>MGSVLSTDSGKSAPASATARALERRRDPELPVTSFDCAVCLEVLHQPVRTRCGHVFCRSCIATSLKNNKWTCPYCRAYLPSEGVPATDVAKRMKSEYKNCAECDTLVCLSEMRAHIRTCQKYIDKYGPLQELEETAARCVCPFCQRELYEDSLLDHCITHHR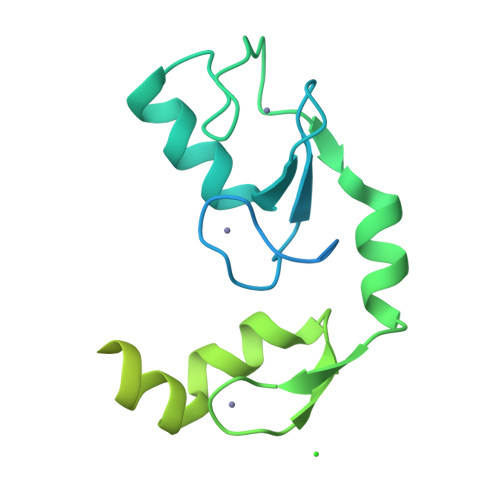SERRPVFCPLCRLIPDENPSSFSGSLIRHLQVSHTLFYDDFIDFNIIEEALIRRVLDRSLLEYVNHSNTT[2x]> PISPIETVPVKLKPGMDGPKVKQWPLTEEKIKALVEICTEMEKEGKISKIGPENPYSTPVFAIKKKDSTKWRKLVDFRELNKRTQDFWEVQLGIPHPAGLKKKKSVTVLDVGDAYFSVPLDEDFRKYTAFTIPSINNETPGIRYQYNVLPQGWKGSPAIFQSSMTKILEPFKKQNPDIVIYQYMDDLYVGSDLEIGQHRTKIEELRQHLLRWGLTTPDKKHQKEPPCLWMGYELHPDKWTVQPIVLPEKDSWTVNDIQKLVGKLNWASQIYPGIKVRQLCKLLRGTKALTEVIPLTEEAELELAENREILKEPVHGVYYDPSKDLIAEIQKQGQGQWTYQIYQEPFKNLKTGKYARMRGAHTNDVKQLTEAVQKITTESIVIWGKTPKFKLPIQKETWETWWTEYWQATWIPEWEFVNTPPLVKLWYQLEKEPIVGAETFYVDGAANRETKLGKAGYVTNKGRQKVVPLTNTTNQKTQLQAIYLALQDSGLEVNIVTDSQYALGIIQAQPDKSESELVNQIIEQLIKKEKVYLAWVPAHKGIGGNEQVDKLVSAGIRHHHHH;> PISPIETVPVKLKPGMDGPKVKQWPLTEEKIKALVEICTEMEKEGKISKIGPENPYNTPVFAIKKKDSTKWRKLVDFRELNKRTQDFWEVQLGIPHPAGLKKKKSVTVLDVGDAYFSVPLDEDFRKYTAFTIPSINNETPGIRYQYNVLPQGWKGSPAIFQSSMTKILEPFKKQNPDIVIYQYMDDLYVGSDLEIGQHRTKIEELRQHLLRWGLTTPDKKHQKEPPFLWMGYELHPDKWTVQPIVLPEKDSWTVNDIQKLVGKLNWASQIYPGIKVRQLSKLLRGTKALTEVIPLTEEAELELAENREILKEPVHGVYYDPSKDLIAEIQKQGQGQWTYQIYQEPF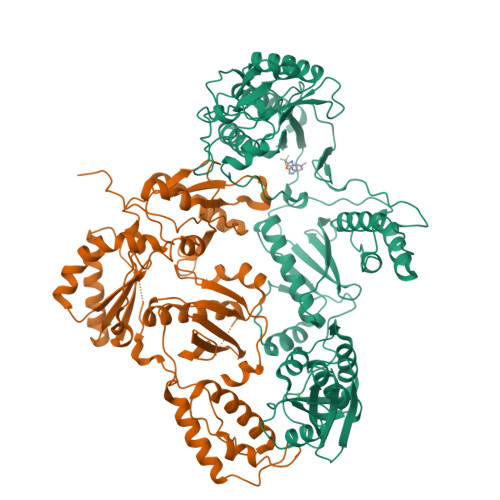KNLKTGKYARMRGAHTNDVKQLTEAVQKITTESIVIWGKTPKFKLPIQKETWETWWTEYWQATWIPEWEFVNTPPLVKLWYQ>[2x]MKMLYDLAKKRKTVRRFKKEKPPLEDLIYSLKVANEAPSGMNAQPWRFLIVEDEKLKGQIRRVCERSEKTFYENVRGRLKEWLDEKRFTWRKPFLKEAP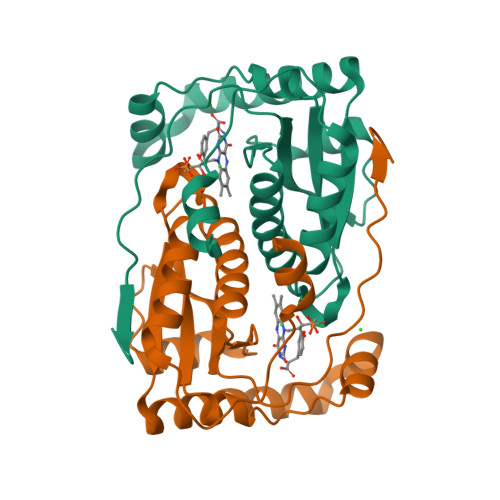YLLLVFSEKSAPYSRESVWLAVGYLLLALEEKGLGSVPYTPPDFREVEKLVNTPSELRLEVILPVGYPDDPKPKYPRNEVIVRYNTFHHHHHH>MGSSHHHHHHSSGLGGTENLYFQSHMDEILARAGIFQGVEPSAIAALTKQLQPVDFPRGHTVFAEGEPGDRLYIIISGKVKIGRRAPDGRENLLTIMGPSDMFGELSIFDPGPRTSSATTITEVRAVSMDRDALRSWIADRPEISEQLLRVLARRLRRTNNNLADLIFTDVPGRVAKQLLQLAQRFGTQEGGALRVTHDLTQEEIAQLVGASR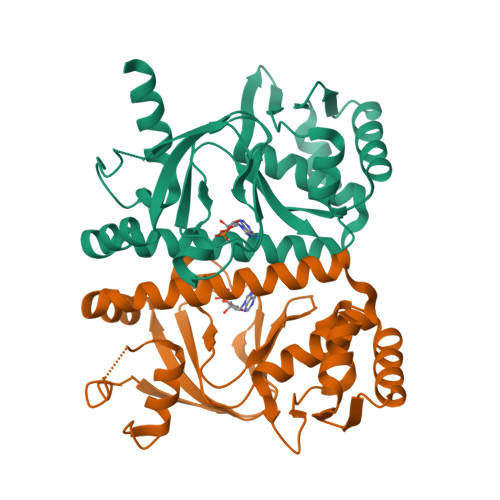ETVNKALADFAHRGWIRLEGKSVLISDSERLARRAR[4x]The bacterial proteins of the Dsb family catalyze the formation of disulfide bridges between cysteine residues that stabilize protein structures and ensure their proper functioning. The oxidative part of this network consists of two monomeric DsbAs (DsbA1 and DsbA2) related to EcDsbL, which cooperate with one DsbB. The solved structures of both CjDsbAs, especially the length and amino acid sequences of their L2 and L3 loops that are essential elements of the monomeric thiol oxidoreductases, were different from that of EcDsbA but similar, though not identical, to that of EcDsbL, which affected their functioning.

CjDsbA1 crystallized in the C2 and P212121 space group containing two monomers in the ASU for the monoclinic form and one molecule per ASU for the orthorhombic form, while CjDsbA2 crystallized in P3221 with a single chain in the ASU. The entire length of the polypeptide could be traced for CjDsbA2, except for the C-terminal HisTag. The active site of CjDsbA1 was observed in the reduced form, while the CjDsbA2 formed a clear disulfide bond. This was due to differences in protein purification procedures. In contrast, the CjDsbA2 experiment was performed under native conditions (without DTT), as the CjDsbA2 reduced form did not bind to the Ni-charged resin. Additionally, the observed effect may have been caused by the prolonged process of CjDsbA2 crystallization (several months) and spontaneous air oxidation or, alternatively, by a photoreduction in CjDsbA1 during X-ray data collection. Redox potentials for both CjDsbA1 and CjDsbA2 were within the limit characteristic for monomeric DsbA oxidative activity (−60 mV for CjDsbA1 and −116 mV for CjDsbA2). We observed that the CjDsbA2 activity in this test was slightly higher than that of CjDsbA1. However, in contrast to CjDsbA1, which in cells lacking its redox partner, was mainly present in a reduced form, the lack of CjDsbB led to almost undetectable levels of CjDsbA2. The extent of CjDsbA2 reoxidation by EcDsbB was rather low, and it did not complement the lack of EcDsbA in either performed test.

> MMEGKEYIILKNPIANADNSLIEIFSYRCTHCYDHHKFNTMGKVKEKLPNLTYKFYPVSSMGDYGRQANEIFAFAAFKDGVNKIDPTDKNSLTHKVAKAYFNAYFKKKQRWENGKNPEAFYSVGLKAMNVSKADLENFLKTPEAAELLKSYEIANPISQNYGTPAFVVNGKYQIIPSAINSPEALIEITKELSKQKLEHHHHHH> NLFQFGDMILQ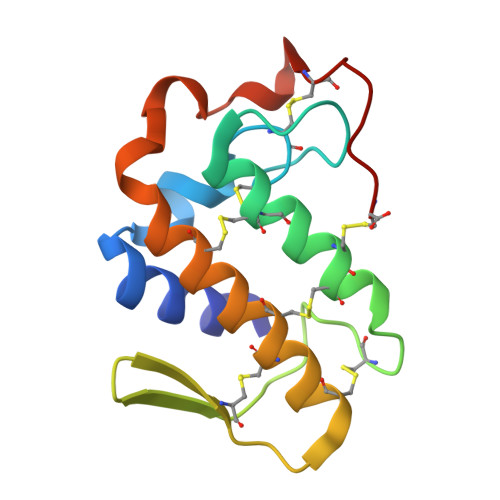KTGKEAVHSYAIYGCYCGWGGQARAQDATDRCCFAQDCCYGRVNDCNPKTATYTYSFENGDIVCGDNDLCLRAVCECDRAAAICLGENVNTYDKNYEYYSISHCTEESEQC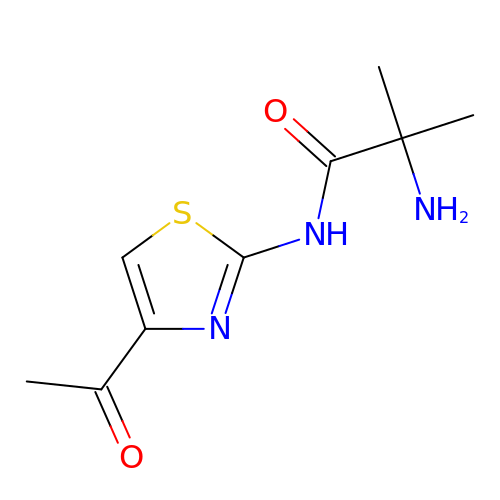2-azanyl-~{N}-(4-ethanoyl-1,3-thiazol-2-yl)-2-methyl-propanamide | C9 H13 N3 O2 S | FFVMFJPYEKSYFF-UHFFFAOYSA-N>[2x]MANSGCKDVTGPDEESFLYFAYGSNLLTERIHLRNPSAAFFCVARLQDFKLDFG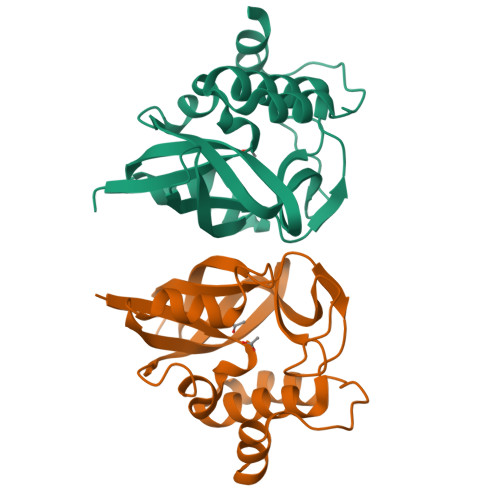NSQGKTSQTWHGGIATIFQSPGDEVWGVVWKMNKSNLNSLDEQQGVKSGMYVVIEVKVATQEGKEITCRSYLMTNYESAPPSPQYKKIICMGAKENGLPLEYQEKLKAIEPNDYTGKVSEEIEDIIKKGETQTL2-IMINO,3-CARBOXY,5-OXO,6-HYDROXY HEXANOIC ACID  | C7 H9 N O6 | 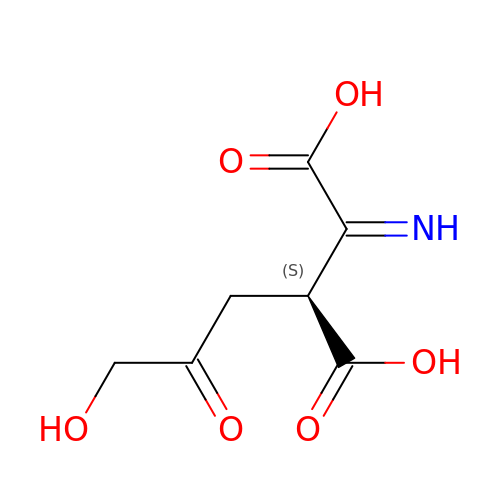RVRAXUFLRLVVQJ-FMAAMLBYSA-N> RSKSSNEATNITPKHNMKAFLDELKAENIKKFLYNFTQIPHLAGTEQNFQLAKQIQSQWKEFGLDSVELAHYDVLLSYPNKTHPNYISIINEDGNEIFNTSLFEPPPPGYENVSDIVPPFSAFSPQGMPEGDLVYVNYARTEDFFKLERDMKINCSGKIVIARYGKVFRGNKVKNAQLAGAKGVILYSDPADYFAPGVKSYPDGWNLPGGGVQRGNILNLNGAGDPLTPGYPANEYAYRRGIAEAVGLPSIPVHPIGYYDAQKLLEKMGGSAPPDSSWRGSLKVPYNVGPGFTGNFSTQKVKMHIHSTNEVTRIYNVIGTLRGAVEPDRYVILGGHRDSWVFGGIDPQSGAAVVHEIVRSFGTLKKEGWRPRRTILFASWDAAEFGLLGSTEWAEENSRLLQERGVAYINADSSIEGNYTLRVDCTPLMYSLVHNLTKELKSPDEGFEGKSLYESWTKKSPSPEFSGMPRISKL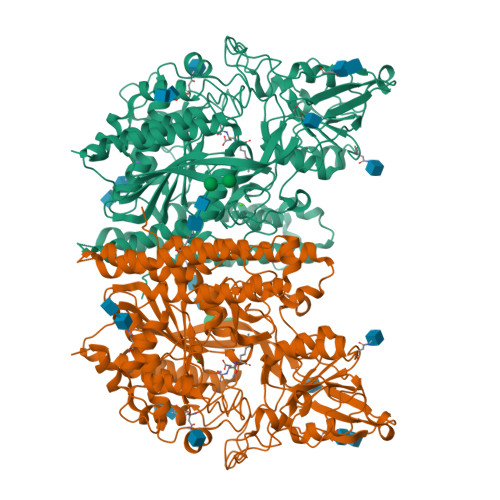GSGNDFEVFFQRLGIASGRARYTKNWETNKFSGYPLYHSVYETYELVEKFYDPMFKYHLTVAQVRGGMVFELANSIVLPFDCRDYAVVLRKYADKIYSISMKHPQEMKTYSVSFDSLFSAVKNFTEIASKFSERLQDFDKSNPIVLRMMNDQLMFLERAFIDPLGLPDRPFYRHVIYAPSSHNKYAGESFPGIYDALFDIESKVDPSKAWGEVKRQIYVAAFTVQAAAETLSEVA> MNKKSIRDVDLKGKRVFCRVDFNVPMKEGKITDETRIRAALPTIQYLVEQGAKVILASHLGRPKGQAVEELRLTPVAARLGELLGKDVKKADEAFGPVAQEMVAAMNEGDVLVLENVRFYAGEEKNDAELAKEFAALADIFVNDAFGAAHRAHASTAGIADYLPAVSGLLMEKELEVLGKALSNPERPFAAIIGGA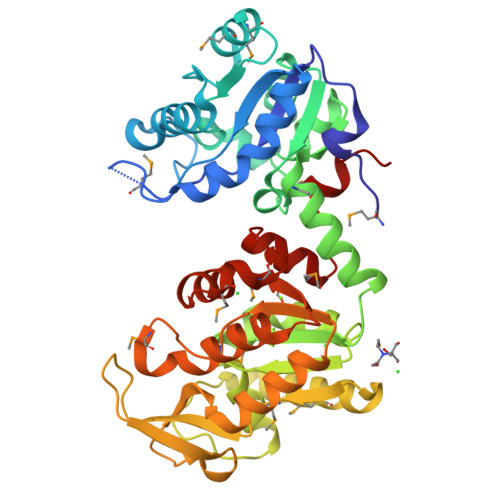KVKDKIGLIRHLLDKVDNLIIGGGLAYTFVKALGHEIGLSLCEDDKIELAKEFMQLAKEKGVNFYMPVDVVITEEFSETATTKIVGIDSIPSNWEGVDIGPKTREIYADVIKNSKLVVWNGPMGVFEMTPFAEGTKAVGQALADAEGTYSVIGGGDSAAAVEKFGMADKMSHISTGGGASLEFMEGKELPGVVCLNDK>[6x]GMSHIQRETSCSRPRLNSNLDADLYGYRWARDNVGQSGATIYRLYGKPNAPELFLKHGKGSVANDVTDEMVRLNWLTAFMPLPTIKHFIRTPDDAWLLTTAIPGKTAFQVLEEYPDSGENIVDALAVFLRRLHSIPVCNCPFNSDRVFRLAQAQSRMNNGLVDASDFDDERNGWPVEQVWKEMHKLLPFSPDSVVTHGDFSL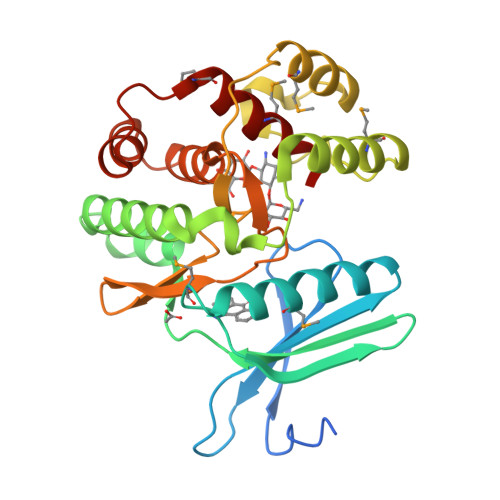DNLIFDEGKLIGCIDVGRVGIADRYQDLAILWNCLGEFSPSLQKRLFQKYGIDNPDMNKLQFHLMLDEFF> SGKVKTGLNSSSSTI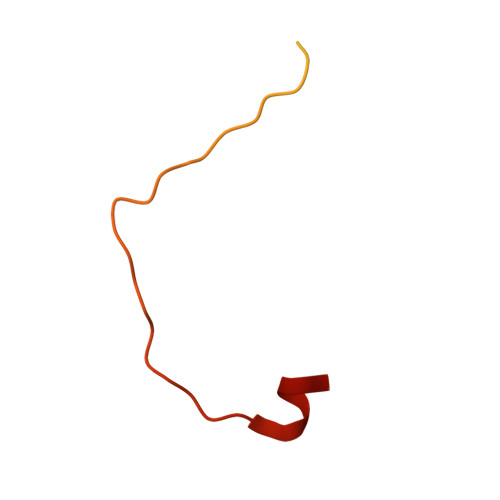DFFKNQYGLLKQTQELEETQKTIGSDETNQADDCNQTVKIWVKYNEGFSNAVRKNVTWNNLWE>GPSGHSARKKPLLQNRHKKARLRFATAHGDKDRTFWRNVLWSDETKIELFGHNDHRYVWRKKGEACKPKNTIPTVKHGGGSIMLWGCFAAGGTGALHKIDGIMDAVQYVDILKQHLKTSVRKLKLGRKWVFQHDNDPKHTSKVVAKWLKDNKVKVLEWPSQSPDLNPIENLWAELKKRVRARRPTNLTQLHQLCQEEWAKIHPNYCGKLVEGYPKRLTQ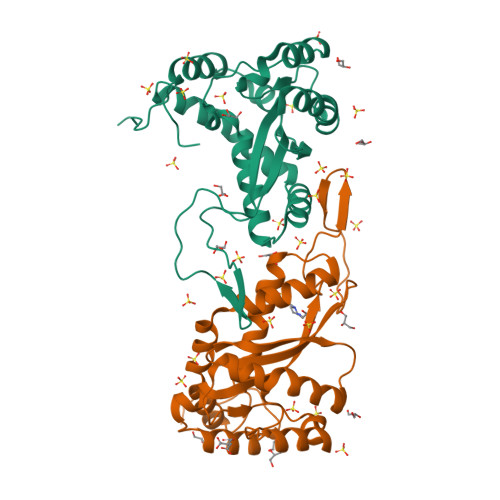VKQFKGNATKY[2x]>[3x]MRLSVCLLMFLLTPIKGDVDSGPPSSATSCKEADMRNSSSEFFNKQWPMPINASKADGIIYPTGKSYSNISLTLQGLFPKHGDLGEQYIYSVGHSDSNYDYLGKLFVSDYATKVVPFNNGFVVRIGAAANATGSVIISTVQKTIKKIYPAFMLGSSVGNFSNGVSGRYFNHTLLLLPDGCGTRLWALYCVIEPRNGSYCPGNSNYNTFAVFDTPHTDCTSAGYNTNATLNSFKEYFDLQNCSFIYSFNITEDENAEWFGITQNTQGVHLYSSRKGDLYGSNMFLFATLPVYDGIKYYTVIPRSIRSKYSERQAWAAFYIYSLHKLTYLLDFSVDGYIRRAVDCGHDDLSQLYCSYESFDVGSGVYSVSSFEVHSRGQFIEQPNSVECDFTKLLSGTPPQVYNFNRLVFTNCNYNLTKLLSLFMVNEFSCDGISPDAIARGCYSSLTVDYFAYPLSMKSYMQPGSAGVISQYNYKQSFANPTCRIFATAPANLTITKPSSYSFISKCSRLTGDNSHIETPIVINPGEYSICKNFAPNGFSQDGDYFTRQLSQLEGGGILVGVGSVTPMTDTLQMGFIISVQYGTDTNSVCPMMDLGNSTTITDKLGVCVEYNLYGVSGRGVFINCTAVGVKQQRFVYDGFDNLIGYYSDDGNYYCVRPCVSVPLSVVYDKTTNSHATIFGSVACEHITTMLHQFSRTTQASLRMRDVSNSGPLQTAVGCVIGLVNSSMVVDNCQLPLGQSLCAVPSTTRSSSQLQLATINYTQPQLLSPLNSSGFVVQVPTNFSFGITQEYIQTTIQKVTVDCKQYVCNGFQKCEQLLREYGQFCAKINQALHGANLMQDESVANLFSDIKTHKSQPLNAGLNGDFNLTLLQVPQVSTSQYSHRSAIEDLLFNKVTIADPGYMQGYDDCMKQGPPSARDLICAQYVAGYKVLPPLYDPNMEGAYTSSLLGSIAGAGWTAGLSSFAAIPFAQSIFYRMNGIGITQQVLSENQKLIANKFNQA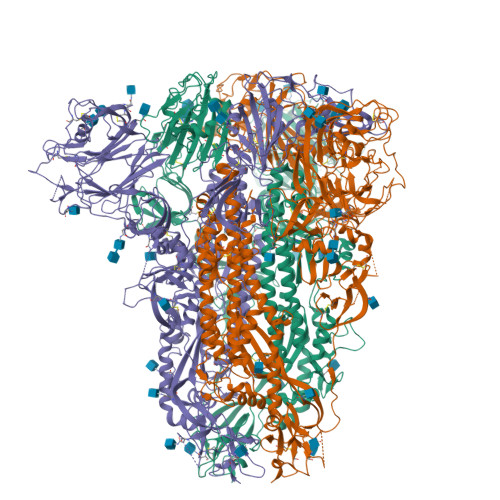LGAMQTGFTTTNLAFSKVQDAVNANAQALSKLASELSNTFGAISSSISDILKRLDAVEQEAQIDRLINGRLTSLNAFVAQQLVRSETAARSAQLASDKVNECVKSQSKRNGFCGSGTHIVSFVINAPNGFYFFHVGYVPTNHVNVTAAYGLCNTDTPPRCIAPIDGYFVLNNTTTRDVVDQWYYTGSSFFNPEPITMANARYVSQDVKFENLTNQLPPPLLNNQTDLDFKEELEEFFKNVSSQGPNFQEISKINTTLLDLSTEMKVLNEVVKQLNESYIDLKELGNYS>MPEIKQLFENNSKWSASIKAETPEYFAKLAKGQNPDFLWIGCADSRVPAERLTGLYSGELFVHRNVANQVIHTDLNCLSVVQYAVDVLQVKHIIVCGHYGCGGVTAAIDNPQLGLINNWLLHIRDYYLKHREYLDKMPAEDRSDKLAEINVAEQVYNLANSTVLQNAW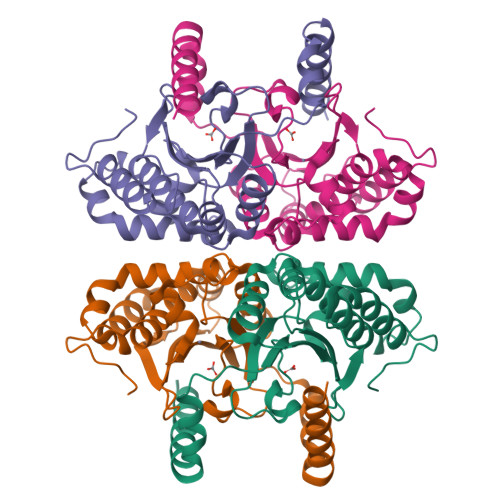ERGQAVEVHGFVYGIEDGRLEYLGVRCASRSAVEDNYHKALEKILNPNHRLLCR[8x]>MFSKFFIERPIFASVVAIIISIAGIIGLANLPVEQYPSLTPPTVQVSATYTGADAQTIASTVATPIEDAINGVDNMIYMDSTSSPGQMKLTVYFNIGTDPDQAAIDVNNRISAATAKLPEAVKKLGVTVRKSSSTILEVVSVYSEDSSMNDIDIYNYVSLNILDELKRIPGVGDASAIGNKNYSMRIWLEPDLLNKFGVTANDVINAVNDQNAQYATGKIGEEPVVNKSPQVISITMQGRLQTPQEFENIILRVNEDKSFLRIKDVAKVEIGAEQYNSTGRLNTSAAVPIIINLQSGANAVNTAKLINEKMQELSKNFPQGLKYQIPYDTTIFVKASIKEVIKTFVEALALVLVVMYLFLKNFKSTIIPMIAVPVSLLGTF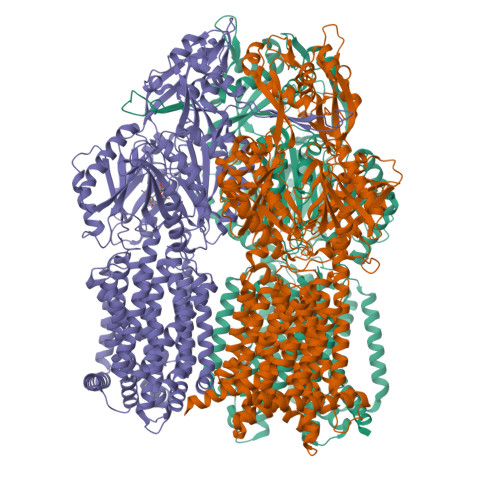AVLYVLGFSINLLTLFALVLAIGIVVDDAIIVVENIDRILHEDSNISVKDAAIKAMNEVSSPVISIVLVLCAVFIPVSFISGFVGEIQRQFALTLAISVAISGFVALTLTPSLSALFLTRNESKPFYFIQKFNDFFDWSTSVFSSGVAYILKRTIRFVLVFCIMIGFIAYLFKIVPSSLVPSEDQGVIMSIINLPSGSSIHRTIEEVDTINKNATQMKEISSSVSLIGFDLFTSSLKENAAAVFFILKDWSQREASSDQIIAQLFGQYAADRNALSYFLNLPPIPGLSLTGGFEMYAQNKSGKDYDAIQQDVNKMLELARTRKELANVRTTLDTSFPQYKLIIDRDKMKYYNLNMQDVFNTISATIGTYYVNDFPMLGKNFQVNIRALGDFRNTQDALKNIYIRSSDNKMIPLNSFLTLVRSAGPDDVKRFNLFPAALIQGDPAPGYTSGQAIDAIAEVAKQSLGDEYSIAWSGSAYQEVSSKGAGAYAFVLGMIFVFLILAAQYERWLMPLAVITAVPFAVFGSILLVALRGFDNDIYFQTGLLLLIGLSAKNAILIIEFAMEERLKKGKSIFEAAINAAKLRFRPIIMTSLAFTFGVLPMIFATGAGSASRHSLGTGLIGGMIAASTLAIFFVPLFFYLLENFNEWLDKKRGKVHE[3x]> MHHHHHHHHAAAGLVPRGSMSQTSTLKGQCIAEFLGTGLLIFFGVGCVAALKVAGASFGQWEISVIWGLGVAMAIYLTAGVSGAHLNPAVTIALWLFACFDKRKVIPFIVSQVAGAFCAAALVYGLYYNLFFDFEQTHHIVRGSVESVDLAGTFSTYPNPHINFVQAFAVEMVITAILMGLILALTDDGNGVPRGPLAPLLIGLLIAVI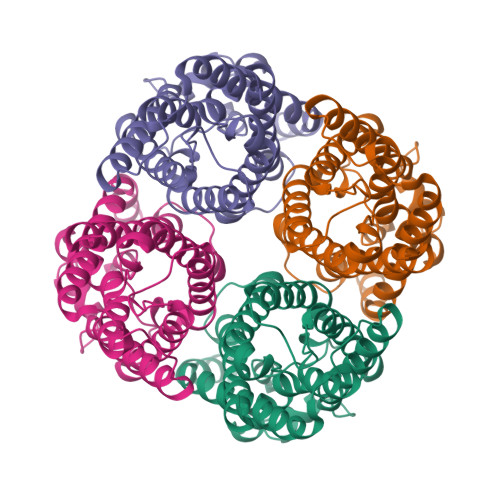GASMGPLTGFAMNPARDFGPKVFAWLAGWGNVAFTGGRDIPYFLVPLFGPIVGAIVGAFAYRKLIGRHLPCDICVVEEKETTTPSEQKASL>[4x]MGSSHHHHHHSQDPGFEFTLMVVGESGLGKSTLINSLFLTDLYSPEYPGPSHRIKKTVQVEQSKVLIKEGGVQLLLTIVDTPGFGDAVDNSNCWQPVIDYIDSKFEDYLNAESRVNRRQMPDNRVQCCLYFIAPSGHGLKPLDIEFMKRLHEKVNIIPLIAKADTLTPEECQQFKKQIMKEIQEHKIKIYEFPETDDEEENKLVKKIKD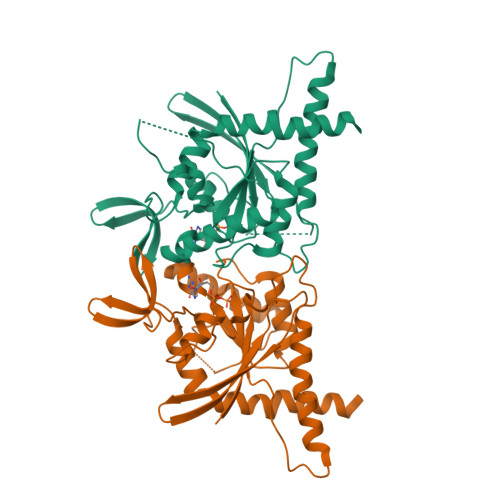RLPLAVVGSNTIIEVNGKRVRGRQYPWGVAEVENGEHCDFTILRNMLIRTHMQDLKDVTNNVHYENYRSRKLAAVT> MAHAGRTGYDNREIVMKYIHYKLSQRGYEWDAGDDVEENRTEAPEGTESEVVHLTLRQAVDDFSRRYRRDFAEMSSQLHLTPFTARGRFATVVEELFRDGVNWGRIVAFFEFGGVMCVESVNR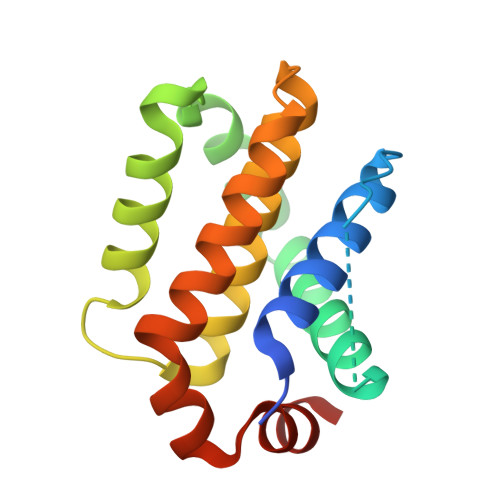EMSPLVDNIALWMTEYLNRHLHTWIQDNGGWDAFVELYGPSMR>[2x]SMAADPQKTAGMRLGNEDFKKDYNIQYAYMTGSMYR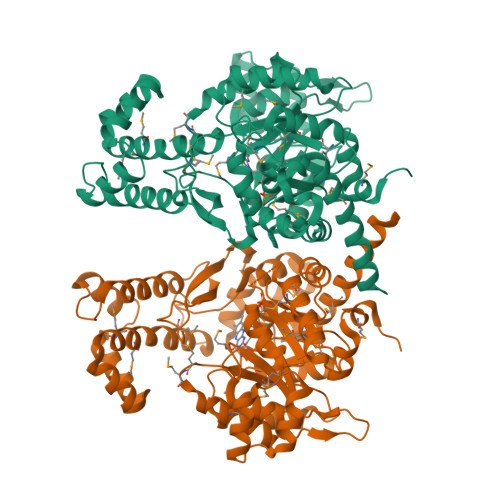GIASEQMVIKAAKAGMLGFFGTGGLSIERIGQAIGTIRSALRQGETFGMNLLHHMMSPDKEVRMIDLYLKNGIHLIEASAFMGITPALVIYRAKGLSRNHDGSVSVQNKIIAKVSRPEVAEAFLNPAPAHVLERLVSDNRLTAGEAALAKEIPMADDICVEADSGGHTDQGIPYTLMPAMIRLRDRMMEKHGYAKKVRIGAAGGIGTPEAAAAAFLLGAEFIGTGSINQCTVEAGTSDSVKDLLQEANVQDTSYAPAGDMFEAGARVQVLKKGLFFPARANKLFDLYRQYNSLDEIDEKTKTLIEEKYFQRSFEEVYEQLKRDKSPEQIAKAEQNPKHKMAMVFKWYFSHTTRLALEGKSESKIDYQIHCGPALGAFNQWVKGTPLENWRNRHVDLIGKQLMEETAGLLAQRLVSITG Rspo (R-spondin, also roof plate-specific spondin) proteins are evolutionarily conserved from fish to humans and have well-documented roles in a broad range of developmental and physiological processes resulting from enhancement of canonical and non-canonical Wnt signalling. ZNRF3/RNF43 specifically targets these Wnt receptors for ubiquitination and turnover, hence reducing Wnt signalling responses. Direct extracellular interaction with Rspo proteins inhibits ZNRF3/RNF43 activity. Here we report a molecular level analysis of the ZNRF3/RNF43 ectodomain structure and its interactions with Rspo proteins.

The crystal structures of the ZNRF3ecto–Rspo2Fu1–Fu2 and RNF43ecto–Rspo2Fu1–Fu2 complexes revealed a 1:1 interaction between Fu1 of the Rspo2Fu1–Fu2 and a single ZNRF3ecto or RNF43ecto chain. The interaction interface between Rspo2Fu1–Fu2 and its two receptors RNF43 and ZNRF3 is essentially the same. It involves an interface area of 990±105 Å2. In contrast, our single structure of RNF43 in complex with Rspo2Fu1–Fu2 displays no dimeric architecture. No dimer is observed in solution for RNF43ecto, even after binding to mRspo2Fu1–Fu2, and we also see only a minor propensity for spontaneous cysteine crosslinking of the P77C (corresponding to S90C of mZNRF3ecto) variant of hRNF43ecto. We note that the residues involved in the dimerization interface of ZNRF3, albeit conserved within the ZNRF3 family, are not conserved between ZNRF3 and RNF43. Furthermore, two glycosylation sites exist in RNF43 and map to the acidic region of the β3–β4 loop and the β1–β2 clamp. These sites are not resolved in the RNF43 complex but might sterically hamper dimerization. However, neither our biophysical measurements nor our structural data for an RNF43 ectodomain in complex with Rspo2 provide any evidence of a similar dimerization mode for RNF43; a finding that argues against ectodomain dimerization having a central role in ligase activity.

> ETGTTEREMDVKALIRVTPLQAEESGGVGQGNLTLEGLFARVAEISPAEGRLLQFHPLSLCNTSEDDQTKPGFISIVKLETPDRDTQPCLSLANKARLAGERGAHAVLFDITNDRGALQQLQQPAGINQPVVLIWGPDAEKLMDVVNKNKEALVKIEVQEQPKWLHHDGTHHHHHHHHHH;> ETGGTNPICKGCLSCSKDNGCLRCQPKLFFYLRREGMRQYGECLQSCPPGYYGVRGPDMNRCSRCRIENCDSCFSRDFCIKCKSGFYSHKGQCFEECPEGFAPLDDTMVCVDGTKHHHHHH>MRILHSMLRVADLEAALEFYTRALDMRL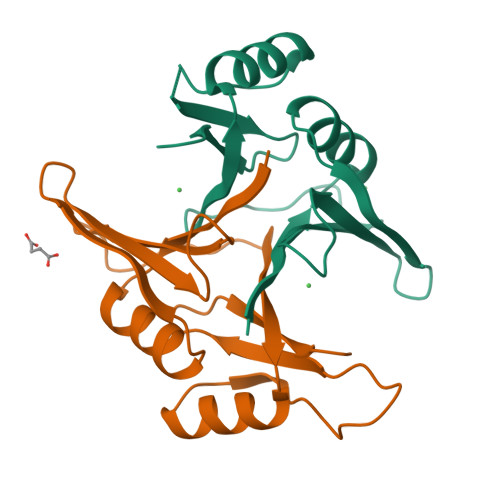LRRRDYPEGRFTLAFVGYQDERAAAALELTHNWDRDGYTQGDGYGHLAIEVEDAAVTCARARALGYRVTREAGLMQHGRSVIAFLEDPDGYKVELIQKGTQFD[2x]>[12x]MIAQGQTLPNATLSQLTKEGMVHHPVLELFAGKKVVLFAVPGAFTPTDSEAHLPGYIVLADQLKAKGVDLIASVSVNDAFVM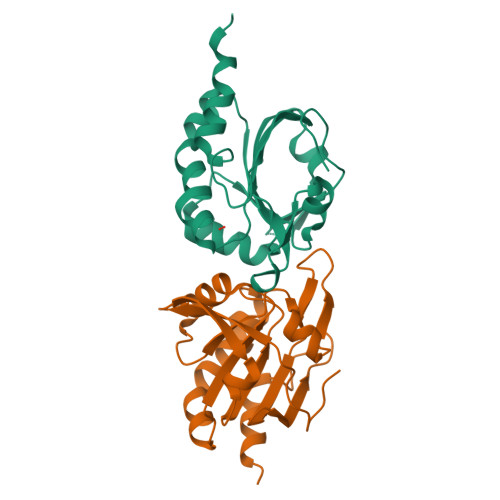KAWGEAQNAEEILMLADGDASFTKALGLEMDTAGFGGLRSQRYAMIIDNGVVTTLNVEAPKSFEVSNAETILAALEHHHHHH> ASSTNLKDILADLIPKEQARIKTFRQQHGNTAVGQITVDMMYGGMRGMKGLVYETSVLDPDEGIRFRGYSIPECQKMLPKAKGGEEPLPEGLFWLLVTGQIPTEEQVSWLSKEWAKRAALPSHVVTMLDNFPTNLHPMSQLSAAITALNSESNFARAYAEGIHRTKYWELIYED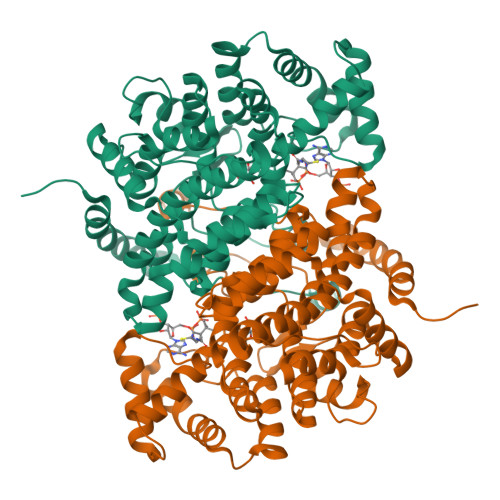CMDLIAKLPCVAAKIYRNLYREGSSIGAIDSKLDWSHNFTNMLGYTDAQFTELMRLYLTIHSDHEGGNVSAHTSHLVGSALSDPYLSFAAAMNGLAGPLHGLANQEVLVWLTQLQKEVGKDVSDEKLRDYIWNTLNSGRVVPGYGHAVLRKTDPRYTCQREFALKHLPHDPMFKLVAQLYKIVPNVLLEQGKAKNPWPNVDAHSGVLLQYYGMTEMNYYTVLFGVSRALGVLAQLIWSRALGFPLERPKSMSTDGLIKLVDSK> PIFLNVLEAIEPGVVCAGHDNNQPDSFAALLSSLNELGERQLVHVVKWAKALPGFRNLHVDDQMAVIQYSWMGLMVFAMGWRSFTNVNSRMLCFAPDLVFNEYRMHKSRMYSQCVRMRHLSQEFGWLQITPQEFLCMKALLLFSIIPVDGLKNQKFFDELRMNYIKELDRIIACKRKNPT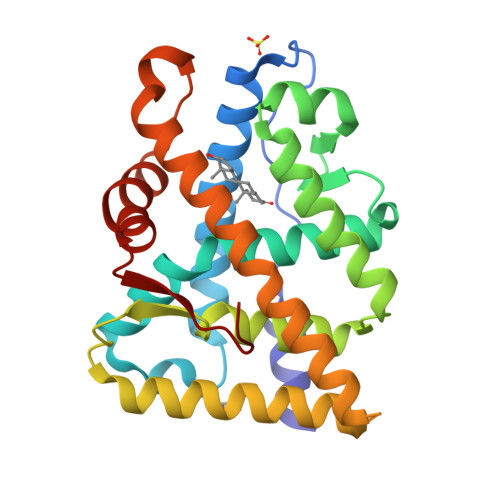SCSRRFYQLTKLLDSVQPIARELHQFTFDLLIKSHMVSVDFPEMMAEIISVQVPKILSGKVKPIYFHTQ>MSDEQKKPEQIHRRDILKWGAMAGAAVAIGASGLGGLAPLVQTAAKPSKKDEKEEEQIVPFYGKHQAGITTAHQTYVYFAALDVTAKDKSDIITLFRNWTSLTQMLTSGKKMSAEQRNQYLPPQDTGESADLSPSNLTVTFGFGPGFFEKDGKDRFGLKSKKPKHLAALPAMPNDNLDEKQGGGDICIQVCADDEQVAFHALRNLLNQAVGTCEVRFVNKGFLSGGKNGETPRNLFGFKDGTGNQSTKDDTLMNSIVWIQSGEPDWMTGGTYMAFRKIKMFLEVWDRSSLKDQEDTFGRRKSSGAPFGQKKETDPVELNQIPSNPHVSLVKSTGKQILRRAFSYTEGLDPKTGYMDAGLLFISFQKNPDNQFIPMLKALSAKDALNEYTQTIGSALYACPGGCKKGEYIAQRLLES[4x]

Bacillus subtilis BsDyP belongs to class I of the dye-decolorizing peroxidase (DyP) family of enzymes and is an interesting biocatalyst due to its high redox potential, broad substrate spectrum and thermostability. DyPs are a family of microbial heme peroxidases that display structural features analogous to chlorite dismutases with an α + β ferredoxin-like fold. In BsDyP, the heme cofactor is partially buried in a predominantly hydrophobic pocket lined by the conserved proximal ligand H326 and catalytic distal residues D240 and R339. Access to the heme from the surface, as defined using a 1.4-Å rolling probe, is made through a distal tunnel and an open wide cavity.

The highest activity for DMP was consistently measured for variant 5G5, which gathered mutations S325P and A330V from variants 1F9 and 3G5, respectively, from the first generation, and mutation K317E from variant 54D6 of the second generation. The variants from the first and second round of evolution, 1F9, 3G5 and 54D6, showed similar kcatapp values for DMP, circa 2-fold of those of the wild type. Noteworthy, the kcatapp of the hit 5G5 variant is ~7-fold higher for DMP, indicating a synergistic action of the three mutations S325P, A330V and K317E in the functional transition. The crystal structure of the 5G5 variant belongs to the monoclinic P21 space group and four monomers in the asymmetric unit were identified. The mutations present in 5G5 are located nearby the heme proximal side. S325P is adjacent to the heme proximal histidine ligand, H326, and mutation A330V lines the cavity at ~3.5 Å to the heme. In the wild-type structure, the side chain of K317 is at the surface, located at ~10 Å from the heme propionate, but in 5G5, E317 is part of a region (309–321) that is not visible in the electron density maps. Therefore, the replacement of K317 with a glutamate disrupted the salt bridge to D250, hypothetically leading to loop 2 destabilization and structural rearrangements that resulted in the higher flexibility of region 309–321. The tunnel that gives access to the heme has a similar length (~10 Å) and diameter (~3 Å) in both the wild type and the 5G5 variant, but the open cavity not only has a higher volume and area, but also an entrance width that is 6 Å larger in 5G5 (~18.0 Å) than in the wild type (~12.0 Å). This results in an increased exposure of the heme group to the solvent: 9% ASA in 5G5 as compared to 4% in the wild type. The results indicate that the variation in the loops’ flexibility and the widening of the active site entrance in the evolved variant 5G5 negatively affect substrate binding, as reflected in higher Michaelis constants, Km, but simultaneously facilitate electron transfer from substrates to the heme, as assessed by the increased catalytic rates of 5G5 for DMP (and also for ABTS).> MSRAKAAPVAGPEVAANRAG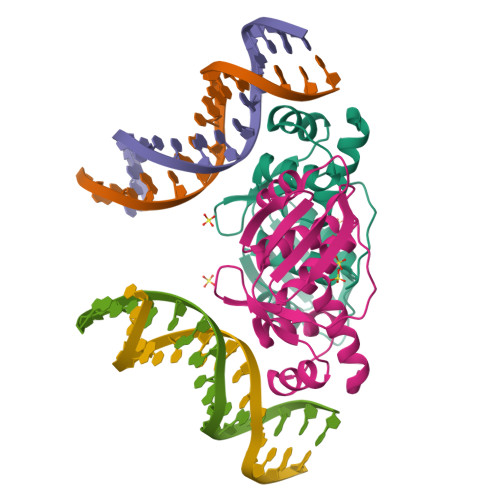RQARIVAILSSAQVRSQNELAALLAAEGIEVTQATLSRDLEELGAVKLRGADGGTGIYVVPEDGSPVRGVSGGTDRMARLLGELLVSTDDSGNLAVLRTPPGAAHYLASAIDRAALPQVVGTIAGDDTILVVAREPTTGAQLAGMFENLR> GAMAGQGDGSVIELGEQTVVATAQEE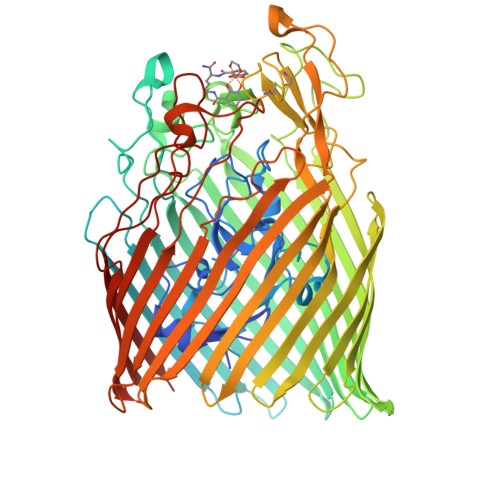TKQAPGVSIITAEDIAKRPPSNDLSQIIRTMPGVNLTGNSSSGQRGNNRQIDIRGMGPENTLILVDGKPVSSRNSVRYGWRGERDSRGDTNWVPADQVERIEVIRGPAAARYGNGAAGGVVNIITKQAGAETHGNLSVYSNFPQHKAEGASERMSFGLNGPLTENLSYRVYGNIAKTDSDDWDINAGHESNRTGKQAGTLPAGREGVRNKDIDGLLSWRLTPEQTLEFEAGFSRQGNIYTGDTQNTNSNNYVKQMLGHETNRMYRETYSVTHRGEWDFGSSLAYLQYEKTRNSRINEGLAGGTEGIFDPNNAGFYTATLRDLTAHGEVNLPLHLGYEQTLTLGSEWTEQKLDDPSSNTQNTEEGGSIPGLAGKNRSSSSSARIFSLFAEDNIELMPGTMLTPGLRWDHHDIVGDNWSPSLNLSHALTERVTLKAGIARAYKAPNLYQLNPDYLLYSRGQGCYGQSTSCYLRGNDGLKAETSVNKELGIEYSHDGLVAGLTYFRNDYKNKIESGLSPVDHASGGKGDYANAAIYQWENVPKAVVEGLEGTLTLPLADGLKWSNNLTYMLQSKNKETGDVLSVTPRYTLNSMLDWQATDDLSLQATVTWYGKQKPKKYDYHGDRVTGSANDQLSPYAIAGLGGTYRLSKNLSLGAGVDNLFDKRLFRAGNAQGVVGIDGAGAATYNEPGRTFYTSLTASF>AKVIFVLAMDVSGKIASSVESWSSFEDRKNFRKITTEIGNVVMGRITFEEIGRPLPERLNVVLTRRPKTSNNPSLVFFNGSPADVVKFLEGKGYERVAVIGGKTVFTEFLREKLVDELFVTVEPYVFGKGIPFF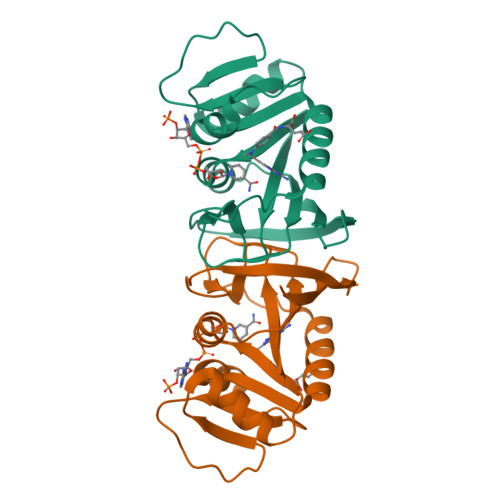DEFEGYFPLKLLEMRRLNERGTLFLKYSVEKSHR[2x]Family 1 glycosidases (GH1) commonly function as β-glucosidases and β-galactosidases, although other activities are also found in the family. GH1 enzymes are present in the three domains of life and have been traced back to LUCA23. We focus on a putative ancestor of modern bacterial and eukaryotic enzymes and find a number of unusual properties that clearly differentiate the ancestor from the properties of its modern descendants. Unexpectedly, the ancestral glycosidase binds heme tightly at a well-defined site in the structure with concomitant allosteric increase in enzyme activity.

Besides interactions with several hydrophobic residues, the bound heme interacts with Tyr264 of α-helix 8 (as the axial ligand), Tyr350 of α-helix 13, Arg345 of β-strand B and, directly via a water molecule, with Lys 261 of β-strand B, although this latter interaction is only observed in chain A. The bound heme shows B-factor values similar to those of the surrounding residues, it is well-packed and 95% buried. Indeed, the accessible surface area of the bound heme is only 43 Å2 compared to the ∼800 Å2 accessible surface area for a free heme. As observed in modern heme-binding proteins, the ancestral heme-binding pocket is enriched in hydrophobic and aromatic residues and propionate anchoring is achieved through interactions with arginine, tyrosine and lysine residues. Heme binding clearly rigidifies the ancestral protein, as shown by fewer missing regions in the electronic density map, in contrast to the structure of the heme-free protein. Lastly, we note that the heme is located near the enzyme active site (at about 8 Å from the catalytic glutamate at position 171) but does not have direct access to this site as revealed in the structure. Therefore, the increase in activity observed upon heme binding is an allosteric effect likely linked to dynamics (see “Discussion”) since heme binding does not substantially alter the position/conformation of the catalytic carboxylic acids nor the residues involved in substrate binding according to the static X-ray structures. The procedure involved in vitro reconstitution using hemin but did not include any chemical system capable of performing a reduction. It is therefore safe to assume that our heme-bound ancestral glycosidase contains iron in the +3 oxidation state. By contrast, heme appears at about 8 Å from the catalytic Glu171 in our ancestral glycosidase.

>MTQTAAKSLKFPKDFLWGAATAAYQIEGAANEDGRGPSIWDTFSHTPGKVHNGDNGDVACDHYHRYKEDVELMKELGLNAYRFSISWPRILPEGEGKVNQKGLDFYNNLIDELLENGIEPFVTLYHWDLPQALQDKGGWENRETVDAFAEYARVCFERFGDRVKYWITFNEPNVFAVLGYLSGVHPPGMKDLKKAFRAAHNLLLAHARAVKAYREISQNGQIGITLNLSPVYPASDNEEEDKAAAERADQFNNWFLDPIFKGKYEHMLERLGEQIAANGGELPEITDEMEILSASLDFIGLNYYTSNLVRANPNSGSSSVKPPDLPRTDMGWEIYPEGLYDLLKRIHEKYNLPIYITENGMAVDDEVEDGAVHDTNRIDYLKEHLEAVHKAIEEGVNVRGYFVWSLMDNFEWANGYSKRFGLIYVDYKTQKRTPKKSAYWYREVIKSNGLELEHHHHHH[3x]> LSCQLY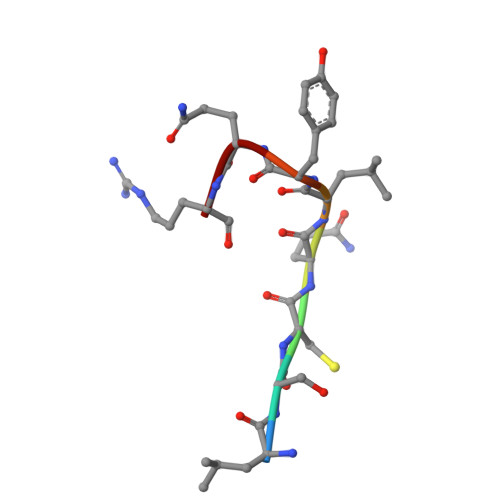QR>MFKDGSLIPYLTAGDPDKQSTLNFLLALDEYAGAIELGIPFSDPIADGKTIQESHYRALKNGFKLREAFWIVKEFRRHSSTPIVLMTYYNPIYRAGVRNFLAAAKASGVDGILVVDLPVFHAKEFTEIAREEGIKTVFLAAPNTPDERLKVIDDMTTGFVYLVSLYGTTGAREEIPKTAYDLLRRAKRICRNKVAVGFGVSKREHVVSLLKEGANGVVV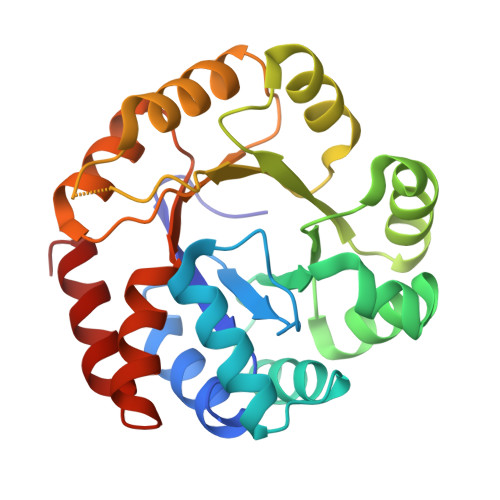GSALVKIIGEKGREATEFLKKKVEELLGI[2x]> GAAEAGITGTWYNQLGSTFIVTAGADGALTGTYESAVGNAESRYVLTGRYDSAPATDGSGTALGWTVAWKNNYRNAHSATTWSGQYVGGAEARINTQWLLTSGTTEANAWKS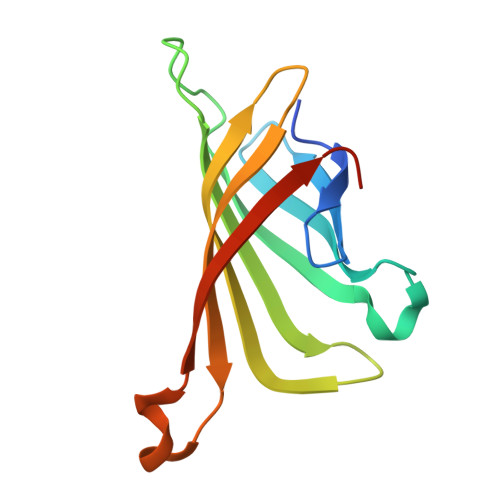TLVGHDTFTKVKPSAAS> CRQKGAGSAGTGSETNSQEVRSQMRSTCLIIPKERFRTMAKEISKKEGHD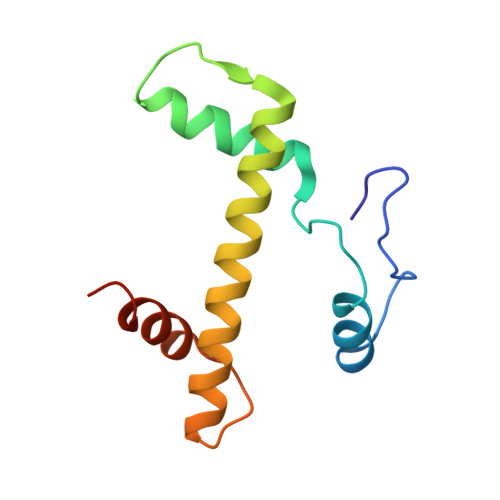VHIAEAALDMLQVIVESCTVRLLEKALVITYSGKRTRVTSKDIETAFMLEHGPLLE>[6x]AAEASKKPRQKRTATKAYNVTQAFGRRGPEQTQGN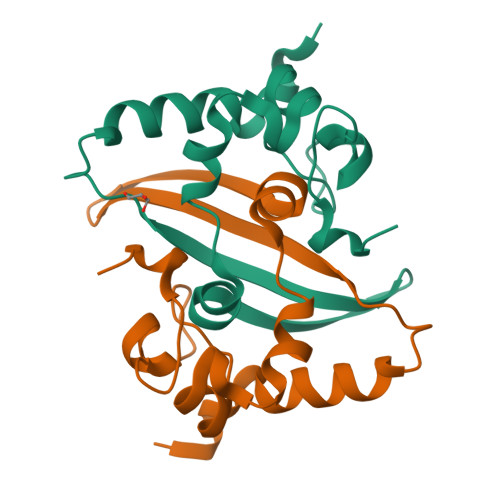FGDQELIRQGTDYKHWPQIAQFAPSASAFFGMSRIGMEVTPSGTWLTYTGAIKLDDKDPNFKDQVILLNKHIDAYKTFP>[2x]GFKQDIATLRGDLRTYAQDIFLAFLNKYPDEKRNFKNYVGKSDQELKSMAKFGDHTEKVFNLMMEVADRATDCVPLASDASTLVQMKQHSGLTTGNFEKLFVALVEYMRASGQSFDSQSWDRFGKNLVSALSSAGMK

Here, a high-throughput approach to determine room-temperature damage-free structures with excellent sample and time efficiency is demonstrated, allowing complexes to be characterized rapidly and without prohibitive sample requirements. We have applied this approach to crystals of two heme peroxidase enzymes: a multifunctional dehaloperoxidase from the marine annelid Amphitrite ornata (DHP-B; Barrios et al., 2014; Franzen et al., 2012; McCombs, Moreno-Chicano, et al., 2017; McCombs, Smirnova et al., 2017) and a dye-decolourizing peroxidase of industrial relevance from Streptomyces lividans (DtpAa). We also examine the challenging case of detecting nitrite binding to copper nitrite reductase from Achromobacter cycloclastes (AcNiR; Horrell et al., 2017), where the ligand displaces a water molecule bound in the active site. Our results cover several different ligand-binding scenarios, such as coordinate-bond formation to a heme iron (imidazole) or copper (nitrite) and noncoordinate ligand binding in a pocket (DHP ligands), with the latter being highly relevant to the binding of ligands to pharmacologically important proteins such as cytochromes P450.

Strong electron-density peaks were present for the two Cl atoms of DCP and the single Br atom of 5BR, allowing the ligand orientation to be easily confirmed, although it is important to note that the electron density was well defined for all atoms of the ligands. For both DHP–ligand structures one monomer had near-full occupancy, but significantly lower occupancy (as refined in PHENIX; Adams et al., 2010) was observed in the second monomer of the homodimer [Figs. 1(a) and 1(b)]. In this case, the lower occupancy of the two 5BR ligands was automatically found in Coot with a data set from 2000 images, but this step failed with 1000 images. A remarkable observation is that even in a data set comprising only 200 images (with 75.3% data completeness) the heavier Br atom of the ligand was clearly identified, with OMIT map peaks of 6.8σ (1.83 e− Å−3) in monomer B and 4.3σ (1.16 e− Å−3) in monomer A at its position. Strong positive density (a 32σ peak) is present where the Br atom of 5BR occupies a similar position to a Cl atom of DCP, consistent with the larger number of electrons on the Br atom. A negative feature is present over the second Cl atom of DCP, consistent with a C atom occupying a similar position in 5BR. Finally, a positive peak is present for the C5 atom of 5BR where no equivalent atom is present in DCP. For example, for the 5BR complex of DHP a subset of just 800 indexed images (∼1.5% of the total number of images in the full data set) was sufficient to correctly model the ligand using a careful strategy to preclude the possibility of model bias.>SNAMLKLGVIGTGAISHHFIEAAHTSGEYQLVAIYSRKLETAATFASRYQNIQLFDQLEVFFKSSFDLVYIASPNSLHFAQAKAALSAGKHVILEKPAVSQPQEWFDLIQTAEKNNCFIFEAARNYHEKAFTTIKNFLADKQVLGADFNYAKYSSKMPDLLAGQTPNVFSDRF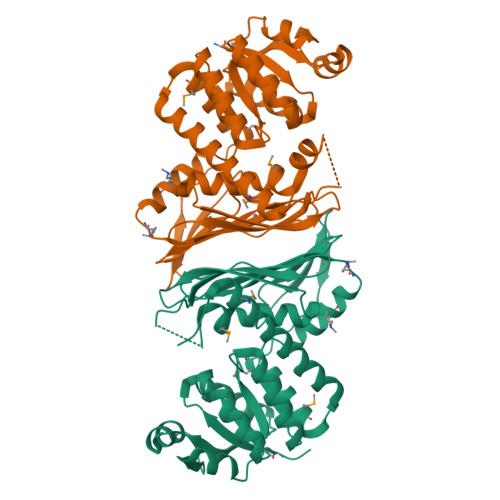AGGALMDLGIYPLYAAVRLFGKANDATYHAQQLDNSIDLNGDGILFYPDYQVHIKAGKNITSNLPCEIYTTDGTLTLNTIEHIRSAIFTDHQGNQVQLPIQQAPHTMTEEVAAFAHMIQQPDLNLYQTWLYDAGSVHELLYTMRQTAGIRFEAEK[4x]4-(2-{[(2-amino-4-methylquinolin-7-yl)methyl]amino}ethyl)-2-methylbenzonitrile | C21 H22 N4 | 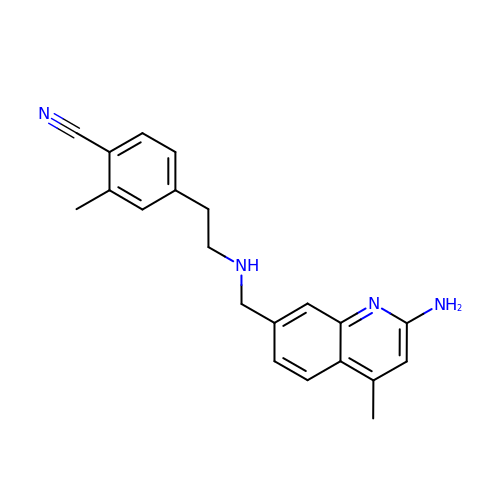GMHLRRHIOCDMQV-UHFFFAOYSA-N> GENIQCGENFMDIECFMVLNPSQQLAIAVLSLTLGTFTVLENLLVLCVILHSRSLRCRPSYHFIGSLAVADLLGSVIFVYSFIDFHVFHRKDSRNVFLFKLGGVTASFTAKVGSLFLAAIDRYISIHRPLAYKRIVTRPKAVVAFCLMWTIAIVIAVLPLLGWNCEKLQSVCSDIFPHIDKTYLMFWIGVVSVLLLFIVYAYMYILWKAGIDCSFWNESYLTGSRDERKKSLLSKFGMDEGVTFMFIGRFDRGQKGVDVLLKAIEILSSKKEFQEMRFIIIGKGDPELEGWARSLEEKHGNVKVITEMLSREFVRELYGSVDFVIIPSYFEPFGLVALEAMCLGAIPIASAVGGLRDIITNETGILVKAGDPGELANAILKALELSRSDLSKFRENCKKRAMSFSDQARMDIELAKTLVLILVVLIICWGPLLAIMVYDVFGKM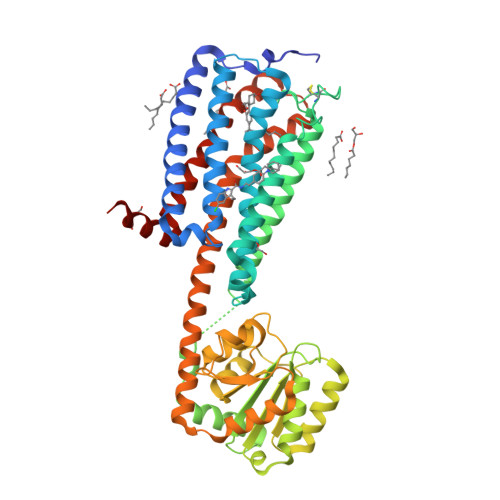NKLIKTVFAFCSMLCLLNSTVNPIIYALRSKDLRHAFRSMFPENLYFQ> MAQHLLHGTLHATIYEVDALHGGGVRQGFLGKILANVEETIGVGKGETQLYATIDLQKARVGRTRKIKNEPKNPKWYESFHIYCAHLASDIIFTVKDDNPIGATLIGRAYIPVDQVINGEEVDQWVEILDNDRNPIQGGSKIHVKLQYFHVEEDRNWNMGIKSAKFPGVPYTFFSQRQGCKVSLYQDAHIPDNFVPRIPLAGGKNYEPQRCWEDIFDAISNAKHLIYITGWSVYAEIALVRDSRRPKPGGDVTIGELLKKKASEGVRVLLLVWDDRTSVDVLKKDGLMATHDEETENFFRGSDVHCILCPRNPDDGGSIVQSLQISTMFTHHQKIVVVDSEMPSRGGSEMRRIVSFVGGIDLCDGRYDTPFHSLFRTLDTVHHDDFHQPNFTGAAITKGGPREPWHDIHSRLEGPIAWDVMYNFEQRWSKQGGKDILVKLRDLSDIIITPSPVMFQEDHDVWNVQLFRSIDGGAAAGFPESPEAAAEAGLVSGKDNIIDRSIQDAYIHAIRRAKDFIYVENQYFLGSSFAWAADGITPEDINALHLIPKELSLKIVSKIEKGEKFRVYVVVPMWPEGLPESGSVQAILDWQRRTMEMMYKDVIQALRAQGLEEDPRNYLTFFCLGNREVKKDGEYEPAEKPDPDTDYMRAQEARRFMIYVHTKMMIVDDEYIIIGSANINQRSMDGARDSEIAMGGYQPHHLSHRQPARGQIHGFRMSLWYEHLGMLDETFLDPSSLECIEKVNRISDKYWDFY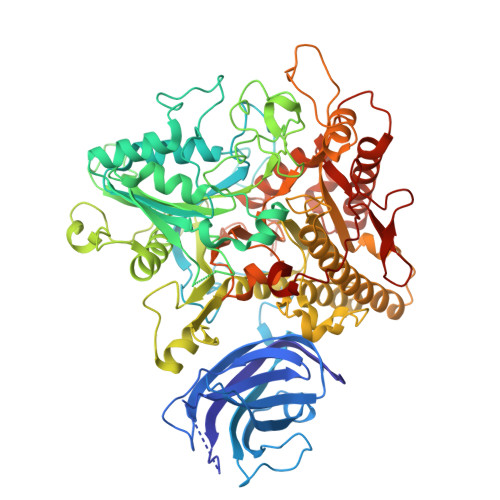SSESLEHDLPGHLLRYPIGVASEGDITELPGFEFFPDTKARILGTKSDYLPPILTT> MKRKLLEILACPLCKSELEVEVVEENEEEIISGKLV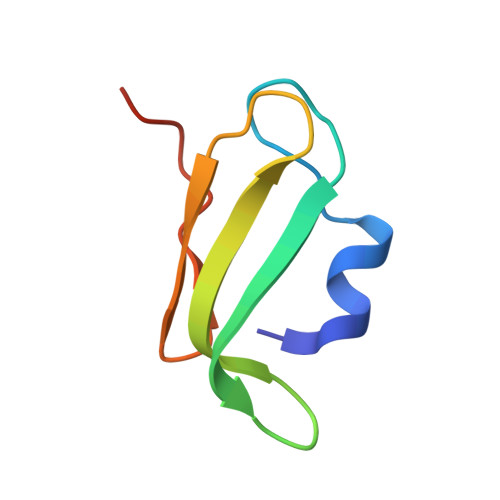CSSCRAEFPIEDGIPDLRPPELRQ>SLKGMISVGPWGGSGGNYWSFKANHAITEIVIHVKDNIKSISFKDASGDISGTFGGKDPRENEKGDEKKIKIHWPTEYLKSISGSYGDYNGVLVIRSLSFITNLTTYGPFGSTSGGESFSIPIADSVVVGFHGRAGYYLDALGIFVQPVPHGTISFGPWGGPAGDDAFNFKVGSWIKDIIIYADAAINSIAFKDANGHCYGKFGGQDPNDIGVEKKVEIDGNLEHLKSISGTYGNYKGFEVVTSLSFITNVTKHGPFGIASGTSFSIPIEGSLVTGFHGKSGYYL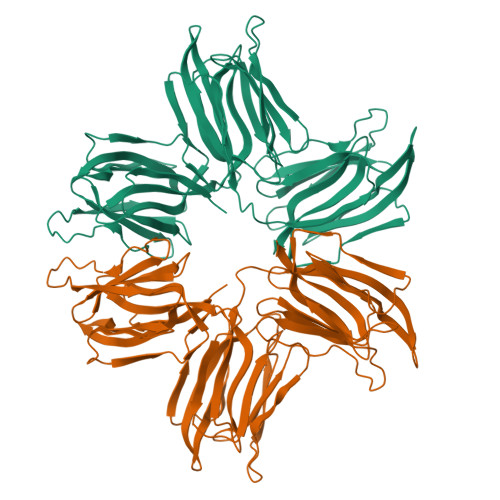DSIGIYVKPRDVEGSISIGPWGGSGGDPWSYTANEGINQIIIYAGSNIKSVAFKDTSGLDSATFGGVNPKDTGEKNTVSINWPSEYLTSISGTYGQYKFKDVFTTITSLSFTTNLATYGPFGKASATSFSIPIHNNMVVGFHGRAGDYLDAIGIFVKPDTAV[2x]1-[4-ethyl-5-[2-[4-[(1-ethylpiperidin-4-yl)methyl]piperazin-1-yl]-1,3-thiazol-4-yl]-2-methyl-1~{H}-pyrrol-3-yl]ethanone 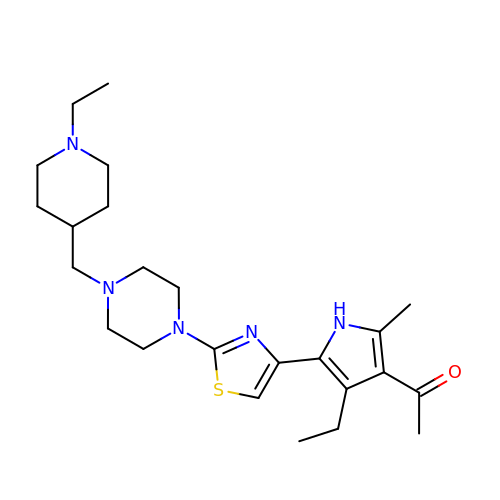| C24 H37 N5 O S | USUFEOMHJBVZED-UHFFFAOYSA-N SusD is an essential component of the sus operon that defines the paradigm for glycan utilization in dominant members of the human gut microbiota. SusD, in association with SusC, a predicted TonB-dependent β-barrel porin, constitutes the minimal starch-binding unit, with further binding affinity provided by SusE and SusF and starch hydrolysis by the α-amylase SusG. BT_3984 is a member of the Pfam SusD/RagB family (PF07980), which includes starch-utilization protein D (SusD) and the immuno­dominant antigen RagB from Porphyromonas gingivalis (note that previous releases of Pfam mistakenly included a reference to a human Ras-related GTP-binding RagB protein that was corrected in the Pfam v.24 release). The SusD protein family (PF07980) contains over 2000 homologs that are predicted to be involved in nutrient binding and whose presence on the outer membrane predisposes them to be effective antigens.

The crystal structure of the Bacteroides thetaiotaomicron protein BT_3984 was determined to a resolution of 1.7 Å and was the first structure to be determined from the extensive SusD family of polysaccharide-binding proteins. At the time of deposition, BT_3984 was the first structural representative of the PF07980 Pfam family of SusD/RagB homologs and belongs to a PUL with unknown specificity and very limited similarity to the archetypal sus operon. The final model includes one BT_3984 molecule (residues 31–537), one acetate molecule, one zinc ion and 705 water molecules in the asymmetric unit. The partially occupied zinc was tentatively assigned based on electron density, coordination geometry and an X-ray fluorescence excitation scan that showed a small peak above background only for zinc. Structural analysis of BT_3984 revealed two tightly packed sub­domains. The N-terminal region consists of three typical tetratrico­peptide repeats (TPRs) that form an αα right-handed superhelix. A mostly unstructured region of ∼100 residues separates the N-­terminal TPRs from a fourth TPR located in the C-terminal region that continues the superhelix. The C-terminal subdomain (residues 266–552) is characterized by a fourth TPR (helices H19–H20) and by long unstructured stretches that comprise over half the sequence of this domain. However, analytical size-exclusion chromatography, in combination with static light scattering, indicates that BT_3984 is likely to be a monomer. By analogy with the conserved TPRs, we propose that these variable TPRs may be involved in binding to more variable members of the SusD-anchored PULs such as, in the case of BT_3984, a predicted uncharacterized glycosyl hydrolase BT_3985.

> GNYENINSNPYEAPDLSADGYALGSAMNNLAGCVVSPDVNTAQFTDCLLGGPLGGYFADSNAGFTETISNFNPKDDWSRVFLKSDKIIPTLYSNLTQVKLVSQNTNDPVPYAIAQVIKVAAMHRVTDAFGPIPYSQIGANGEIATPYDSQEVTYNTFFDELNAAIATLNENSNEQLVPTADYIYKGDVKKWIRFANSLKLRLAIRIAYANPVKAQQMAEEAVNPANGGVIESNADNATWNYFETSQNPIYVATRYNQVQTSDHGGVPCLTGGDTHAAADIICYMNGYKDNRREKFFTKSEWAGQDYVGMRRGIVIPELKTTGHKYSGVNIAPTSPLYWMNAAEVAFLRAEGQAVFNFSMGGTAESFYNQGIRLSFEQWGADGVEDYLKDDVNKPTAYTDPAGTNTYQNALSNITIKWNDSADKEEKQERIIVQKWIANWQLGNEAWADFRRTGYPKLIPVKENKSGGVVDSEKGARRMPYPLDEFVSNKANVEYAIANYLHGADNMATDVWWASKK> KETAAAKLERQHLDS;> NYCNQ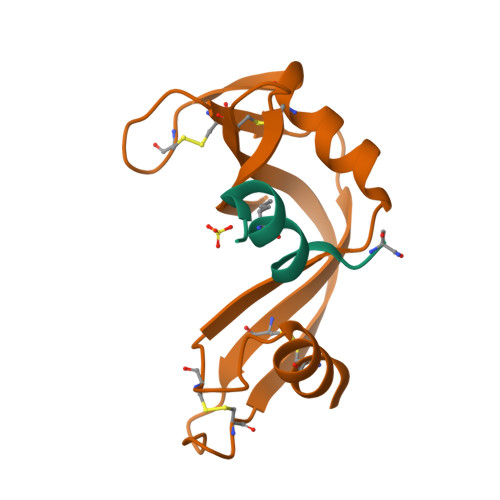MMKSRNLTKDRCKPVNTFVHESLADVQAVCSQKNVACKNGQTNCYQSYSTMSITDCRETGSSKYPNCAYKTTQANKHIIVACEGNPYVPVHFDASV> MERTVVETRYGRLRGEMNEGVFVWKGIPYAKAPVGERRFLPPEPPDAWDGVREATSFGPVVMQPSDPIFSGLLGRMSEAPSEDGLYLNIWSPAADGKKRPVLFWIHGGAFLFGSGSSPWYDGTAFAKHGDVVVVTINYRMNVFGFLHLGDSFGEAYAQAGN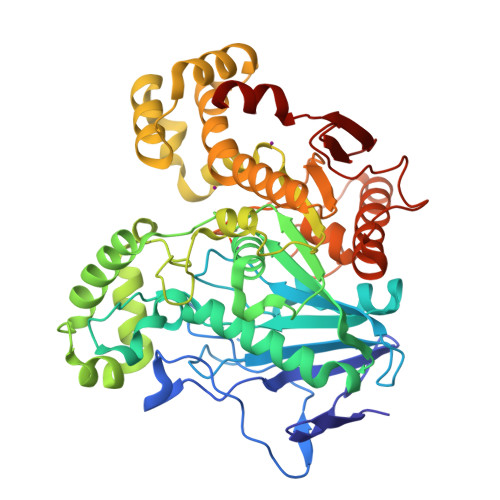LGILDQVAALRWVKENIAAFGGDPDNITIFGESAGAASVGVLLSLPEASGLFRRAMLQSGSGSLLLRSPETAMAMTERILDKAGIRPGDRERLLSIPAEELLRAALSLGPGVMYGPVVDGRVLRRHPIEALRYGAASGIPILIGVTKDEYNLFTLTDPSWTKLGEKELLDRINREVGPVPEEAIRYYKETAEPSAPTWQTWLRIMTYRVFVEGMLRTADAQAAQGADVYMYRFDYETPVFGGQLKAAHALELPFVFHNLHQPGVANFVGNRPEREAIANEMHYAWLSFARTGDPNGAHLPEAWPAYTNERKAAFVFSAASHVEDDPFGRERAAWQGR> SNAMPSAMNERTVAELEK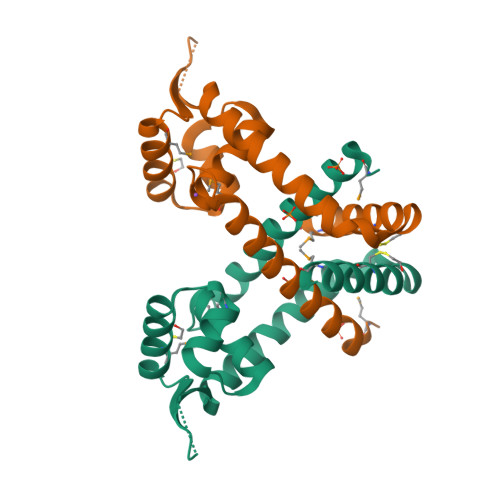LLRYIAANLKQRGREILTNYPITPPQFVALQWLLEEGDLTVGELSNKMYLACSTTTDLVDRMERNGLVARVRDEHDRRVVRIRLLEKGERIIEEVIEKRQRDLANVLESFSDEEIVVFERCLRKLHQEMTKE>[60x]MNNLYRDLAPITESAWAEIELEATRTFKRHIAGRRVVDVSGPNGPTTASVSTGHLLDVSPPGDGVIAHLRDAKPLVRLRVPFTVARRDIDDVERG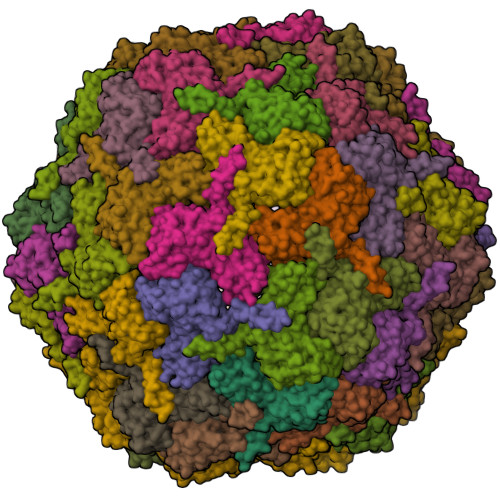SQDSDWDPVKDAAKKLAFVEDRAIFEGYAAASIEGIRSSSSNPALALPDDAREIPDVIAQALSELRLAGVDGPYSVLLSAETYTKVSETTAHGYPIREHINRLVDGEIIWAPAIDGAFVLSTRGGDFDLQLGTDVSIGYLSHDAEVVHLYMEETMTFLCYTAEASVALTPELWSHPQFEK>[8x]MAEGERQPPPDSSEEAPPATQNFIIPKKEIHTVPDMGKWKRSQAYADYIGFILTLNEGVKGKKLTFEYRVSEAIEKLVALLNTLDRWIDETPPVDQPSRFGNKAYRTWYA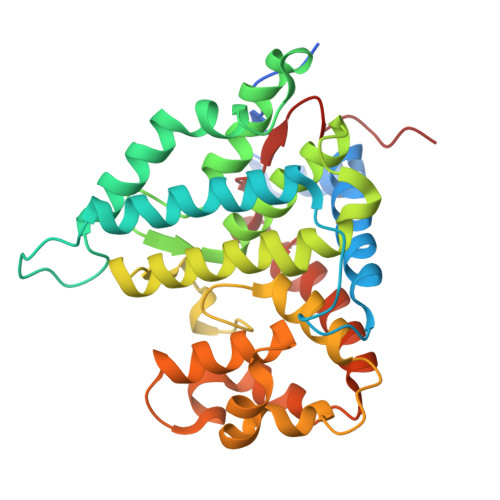KLDEEAENLVATVVPTHLAAAVPEVAVYLKESVGNSTRIDYGTGHEAAFAAFLCCLCKIGVLRVDDQIAIVFKVFNRYLEVMRKLQKTYRMEPAGSQGVWGLDDFQFLPFIWGSSQLIDHPYLEPRHFVDEKAVNENHKDYMFLECILFITEMKTGPFAEHSNQLWNISAVPSWSKVNQGLIRMYKAECLEKFPVIQHFKFGSLLPIHPVTSG> EFKLSEGQRAIYNFHKKVRKDVKNCRIPGQPPAKNLTKLKWNKLLANKAKQQAKRCKYDSNDPNDFIIGDFESIGQNLADYPTIEGAMKDWLEEYKNYNFEKNQCNGDCKNYKQMVWNTTEEIGCGYEKCGKNYLIVCNYAPGDSEDRPYEAKPESKCNKSE

Vaccine candidates have been identified, including Schistosoma mansoni venom allergen-like proteins (SmVALs) from the SCP/TAPS (sperm-coating protein/Tpx/antigen 5/pathogenesis related-1/Sc7) superfamily. SmVALs are characterized by a single CAP domain otherwise referred to as SCP/TAPS, NCBI domain cd00168 or Pfam PF00188, which is found in diverse unrelated proteins from bacteria, plants, animals and viruses. SmVAL4 is secreted at stages linked to invasion, which makes it a viable choice as a vaccine candidate. The expression of SmVAL4 by yeast cells lacking endogenous CAP function restores the block in sterol export. These studies suggest an evolutionarily conserved lipid-binding function for CAP or SCP/TAPS proteins, including SmVAL4 and yeast Pry1.

The structure of the first SCP/TAPS protein from a schistosome has been refined to 2.16 Å resolution. The refined model has one monomer of SmVAL4 in the asymmetric unit. The recombinant protein is N-glycosylated and is a monomer in solution, unlike some other reported CAP or SCP/TAPS proteins such as NaASP2, GAPR-1, VesV5 and GLIPR-1, which were shown to form dimers. SmVAL4 retains the characteristic α/β sandwich CAP structure and a large central cavity. SmVAL4 has unique loop regions, including a C-terminal extended loop with a terminal helix. Only the CAP4 motif is present in SmVAL4 and the CAP cavity of SmVAL4 lacks all but one of the signature CAP cavity tetrad amino-acid residues. The absence of these histidines makes SmVAL4 incapable of coordinating Zn2+ and implies different underlying mechanisms for the function of SmVAL4, independent of these residues; indeed, these residues were shown to be unnecessary for sterol transport in yeast CAP proteins. A similar cavity was observed between the corresponding α-helices 1 and 4 in the SmVAL4 structure. While the residues are not conserved across the representative CAPs, there is sufficient space between the equivalent helices to facilitate palmitate binding. These analyses reveal that SmVAL4 is structurally able to accommodate lipids such as palmitate, and it is possible that palmitate binding in SmVAL4 is akin to what was observed for tablysin-15. While we show that SmVAL4 is capable of binding lipids, the electron-density maps do not show any evidence of any bound lipid.TMEM106B is a type II transmembrane protein of 274 residues that localizes to late endosomes and lysosomes. Here we used structure determination by cryogenic electron microscopy to show that residues 120–254 of the lysosomal type II transmembrane protein 106B (TMEM106B) also form amyloid filaments in human brains. The TMEM106B folds shared a similar five-layered ordered core comprising residues S120–G254 and contained 17 β-strands, each ranging between 3 and 15 residues. We observed three TMEM106B folds, with no clear relationships between folds and diseases.

Our best maps for filaments with folds I, II and III had resolutions of 2.6, 3.4 and 2.8 Å, and came from case 1 (sporadic Alzheimer’s disease), case 19 (MSA) and case 17 (MSA), respectively. For all three folds, we determined the structures of filaments that were made of a single protofilament. In fold I, this region packs loosely against the other side of the C-terminal hairpin-like region with the formation of three large amphipathic cavities. Likewise, there is an extra density in front of the side chain of Y209 in fold I, but not in the other folds. Individuals with fold I were homozygous for T185 or S185, or heterozygous, indicating that fold I can accommodate a threonine or a serine at position 185. Owing to the compatibility of both residues with the glycosylation motif at N183, no differences in the associated glycan densities were observed. Filaments with fold I were more common than filaments with folds II or III. We divide the sequence that forms the ordered cores of the folds into three regions according to their degree of structural conservation: the amino-terminal region (S120–T166) is conserved in all three folds; the C-terminal region (Y211–G254) is conserved only in folds I and II; and the middle region (A167–M210) varies between folds.

>[3x]MGKSLSHLPLHSSKEDAYDGVTSENMRNGLVNSEVHNEDGRNGDVSQFPYVEFTGRDSVTCPTCQGTGRIPRGQENQLVALIPYSDQRLRPRRTKLYVMASVFVCLLLSGLAVFFLFPRSIDVKYIGVKSAYVSYDVQKRTIYLNITNTLNITNNNYYSVEVENITAQVQFSKTVIGKARLNNISIIGPLDMKQIDYTVPTVIAEEMSYMYDFCTLISIKVHNIVLMMQVTVTTTYFGHSEQISQERYQYVDCGRNTTYQLGQSEYLNVLQPQQ>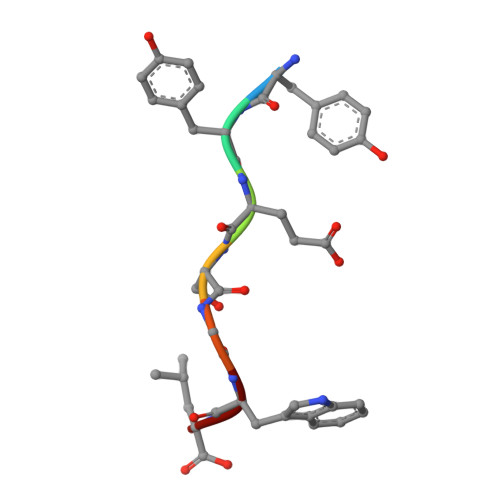 YYESGWL>[2x]GPGSMAATIRYHEGDISAEDAARYKGAIAIDTETLGLVPRRDRLCVVQLSSGDGTADVI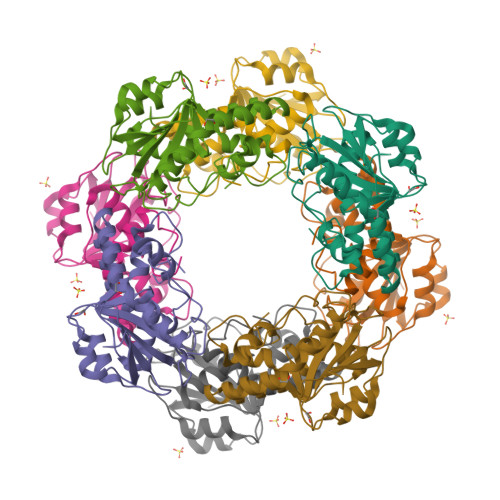RIAAGQKQAPNLVHMLADPARQKIFHYGRFDIAVLFHTFGVTTTPVFCTKIASRLCRTYTDRHGLKDNLKEMLEVDISKAQQSSDWAAETLSPAQLEYAASDVLYLHALRDKLTARLIRDGRIEHADACFAFLPTRAKLDLLGWDETDIFAHS> MGSSHHHHHHSQDPMEIDELTALGGLLHDIGKPVQRAGLYSGDHSTQGARFLRDLAENTGRAEYELLSLFSEFHHKGHMKNDELMIRRIKELSPERFGLTMEDVLNALWIVYEADNLASGEREEGQPQASRPLYSVFNPGKAYPWAELDFEKELPVPGDVFSIRSQDYRELVKRLWEELSKAKLRSDRLLPVLEKYLTFVSSVTSEGNIISLYDHMRMTSAIALAMLRAGCTAEDVRSGRCRKEKRFLLIEGDFSGIQDFIYRVSGKGTLKYLRARSAYLELIGWDVVLEILSRLGLTRANVVFNAGGHFMIIAQNTPDAVKELEEIRAKAVEWLYREFESDLYLAIEWEPVSGREFGREGGKNLFAEARKRLKHKLTVRKLKRFGEIKGLFEHGHTERLAECPVCGRELPEGKLEPSASDPETKVCPTCNRLVSLGGNLPKLLGFGRTAKNDAGVLVEGPFSGFVPYLQGGRPVGEQILVKNTLNPGEIPESAQFVPYFVA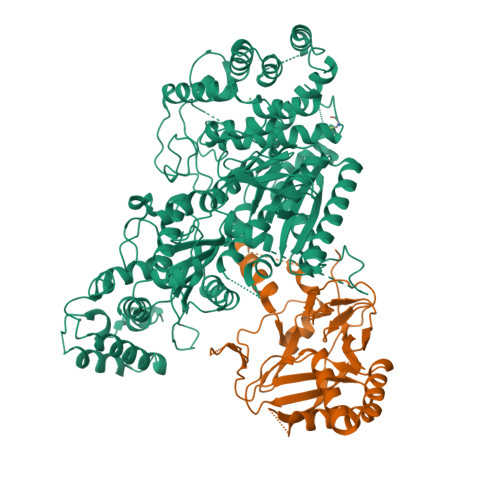DYFKKDPKGGVATFEELSMASTGTRRLGVMKGDVDRLGEFFSSMDSPSKLATASRFMDYFFKGYIGAIIEGKFGYIIGDVPSLRDWPEEPDIVVVYAGGDDFFIVGAWDQIFELAFRVRRAFNAYTGGKLTLSVGLGYFDERTPIYRMADVVSERLDTAKDEGRNRVFVVGRSRPLDGKHKLSYEWNHYEELWRTYAPRIYAGNGRLKGKLESKKGLLWKLLEIRELYVRDPNDVRWAYLTAYLLGRHGLSDLFPELVGIDTKAVERKEPQPVYWVDGVLKIVLMAVRR;> MPKFIAVKLIPKGPFRDIPRADTLFGAIGNAISAIHGQSAVEELVDAFVGGARISSAFPYSGDTYYLPKPLSVEPALEGILTGLDEEERYTTAKRLRKAKYLDLKNFELALRLRPFTIPEEIPYARVDVPRVVLDRVTQDSSIYFWEEIRFREKSGVYFLYSGPREVFDGYIAPAMRFLGDTGIGGKSTWGAGLFEVEFHEMKIDAPGSEYSVTLSNALPTKTPVLWRLLRKGGWSFGRRKPRMTFIAEGSIVKNDPGGMERLELGLSHEVYVYGLTFPLGVELPEGLE Milano is a contractile tail bacteriophage that infects the pathogenic plant bacterium Agrobacterium tumefaciens, an important tool that is widely used in genetic manipulations of plants. The contractile tail of Agrobacterium tumefaciens bacteriophage Milano is flexible and bent to varying degrees, which sets it apart from other contractile tail-like systems. A contractile sheath and rigid tube assembly is a widespread apparatus used by bacteriophages, tailocins, and the bacterial type VI secretion system to penetrate cell membranes. In this mechanism, contraction of an external sheath powers the motion of an inner tube through the membrane.

In the initial extended (pre-attachment) conformation, virtually all tails in cryo-EM images were bent, complicating the reconstruction procedure. The curved tail structure was reconstructed by dividing the tail into overlapping segments. Fragments with a common curvature were clustered using 3D variability analysis and used for reconstruction with no symmetry imposed. As a result, the surface of the tube displays substantial grooves at the interface of two rings that are not found in straight tubes of other CIS. In the curved tail, these grooves are smaller on the inner surface of the curve when compared to the straight state, showing that these grooves enable the bending. The backbone traces of the tube subunit in the baseplate-proximal straight region and in the curved middle region of the Milano tail structure are virtually identical with an RMSD value between their Cα atoms of ~0.5 Å which is at the level of experimental error. The curvature is therefore realized at the level of side chains, which adopt slightly different conformations in the grooves separating the subunits. The interactions of sheath and tube subunits in straight and curved tail segments are very similar, suggesting that these interactions do not constrain the bending. In the extended tail, these charges are neutralized by the sheath (specifically, by the SHD), and the tube-sheath assembly is flexible. The cryo-EM map shows that each sheath-subunit forms three different disulfide bonds with neighboring subunits, covalently linking all subunits together.

>MACNKQNGVKNILITFTDCDTQEVIGPISHEQPDDTLPTYKNCAWTNTALTNGYVQRSASNATMTLPVVRDLRVPLAFYQGCAQVDVQVEKFDGTVMTLTEGAVVEPEESDGRSVTMNIVASEIDELLPPGSLAAA[18x];>[12x]MAQDALSDGFVRLCIDPSLNFFGEGCKILVEGQMTDDGSATPDAVTCVTSELDIIERFGQGSVLTESLRKVFCTCKSGVSVYALPREDAAAGVKAVYTLTIAGPATTDGRVQLYMGEAEYAVDIGVDAGDTATDIAAAIVAAISPDFPYAATAAAGVITLTARNAGTIGNHLSVIYTNLGSCTSVTPEGVTVTFAQTTAGSVNPTPNDYATVVNECCFAVYVLSSDDTDWQENLRDWIRSAWDCSKPQCFGHGYVFNKGTLGQVLADGDNSAELSRLALPTTYPVLPYLTNAAYGALSACSTCNNPELNIQGQTFGLLSCINMPESCTPGWTFGEVTQLQANGFVVSGPSTTSGQGNYTSPYIYNDVTNYLRDEKNRPNATFRDASSRRLAAATGVALAEFLQQFNGLAVFTKNTNIRTGIIGTNPRLMLGKIRKWAQDNVGTLFSEFDNINEDIQLLTDFEVQPKCVGQPGIFHLNMRYRPPVRGARINVNMAPALFDNCDR>MHHHHHHHMSKAFIGKPAPDFATKAVFDGDFVDVKLSDYKGKYVVLFFYPLDFTFVCPTEIIAFSDRFPEFKNLNVAVLACSTDSVFSHLAWINTPRKHGGLGDMKIPVLADTNHQIAKDYGVLKDDEGIAYRGLFIIDPKGILRQITINDLPVGRSVDETLRLVQAFQYTDKHGEVCPAGWT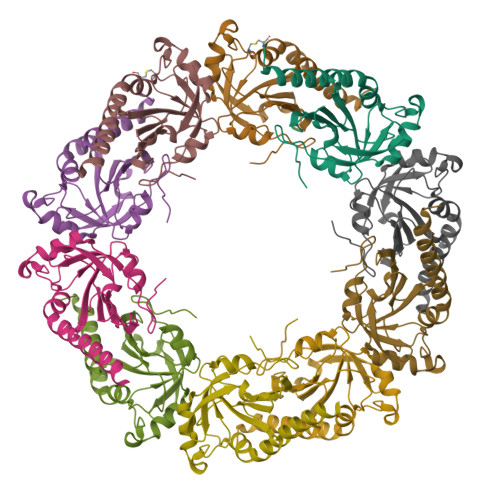PGKDTIKPAVKESKEYFNKAN[10x]5-{[(2S)-2-cyclopropyl-7,8-dimethoxy-2H-chromen-5-yl]methyl}pyrimidine-2,4-diamine 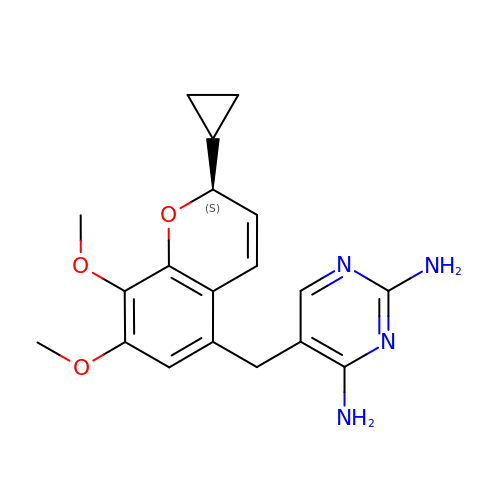| C19 H22 N4 O3 | HWJPWWYTGBZDEG-CQSZACIVSA-N2-[2-(2-chlorophenyl)sulfanylethanoyl-[[4-(1,2,4-triazol-1-yl)phenyl]methyl]amino]-N-methyl-ethanamide 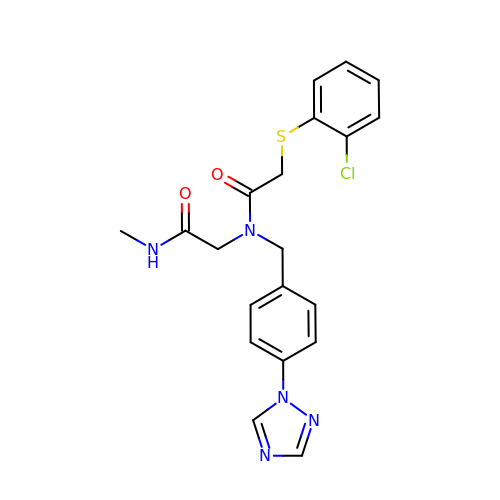| C20 H20 Cl N5 O2 S | NVGPCILMXWWONB-UHFFFAOYSA-N> MEGQGCCGGGGGKTEMI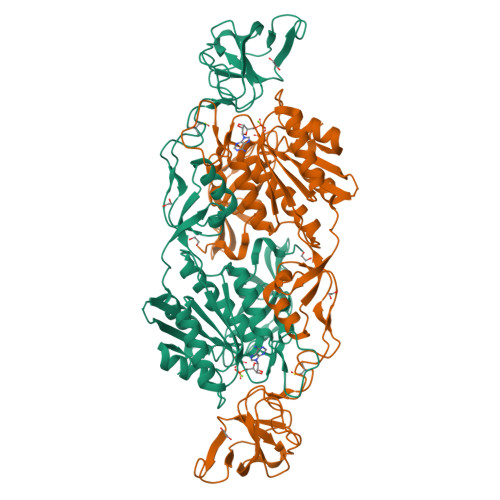PTEEALRIVFGVSKRLPPVIVSLYEALGKVLAEDIRAPDPLPPYPASVKDGYAVVASDGPGEYPVITESRAGNDGLGVTVTPGTVAYVTTGGPIPDGADAVVQVEDTKVIGDVSTESKRVKILIQTKKGTDIRRVGCDIEKDATVLTTGERIGASEIGLLATAGVTMVKVYPMPIVAILSTGDELVEPTAGTLGRGQIRDSNRAMLVAAVMQQQCKVVDLGIVRDDRKELEKVLDEAVSSGVDIILTSGGVSMGDRDFVKPLLEEKGKVYFSKVLMKPGKPLTFAEIRAKPTESMLGKTVLAFGLPGNPVSCLVCFNIFVVPTIRQLAGWTSPHPLRVRLRLQEPIKSDPIAPEFHRAIIKWKDNDGSGTPGFVAESTGHQMSSRLLSMRSANALLELPATGNVLSAGSSVSAIIVSDISAFSIDKKASLSEPRSWSHPQFEK>GQPPRRYTPDWPSLDSRPLPAWFDEAKFGVFIHWGVFSVPAWGSEWFWWHWQGEGRPQYQRFMRDNYPPGFSYADFGPQFTARFFHPEEWADLFQAAGAKYVVLTTKHHEGFTNWPSPVSWNWNSKDVGPHRDLVGELGTALRKRNIRYGLYHSLLEWFHPLYLLDKKNGFKTQHFVSAKTMPELYDLVNSYKPDLIWSDGEWECPDTYWNSTNFLSWLYNDSPVKDEVVVNDRWGQNCSCHHGGYYNCEDKFKPQSLPDHKWEMCTSIDKFSWGYRRDMALSDVTEESEIISELVQTVSLGGNYLLNIGPTKDGLIVPIFQERLLAVGKWLSINGEAIYASKPWRVQWEKNTTSVWYTSKGSAVYAIFLHWPENGVLNLESPITTSTTKITMLGIQGDLKWSTDPDKGLFISLPQLPPSAVPAEFAWTIKLTGVK[4x]

In humans, the dynamic process of α-L-fucose removal is catalyzed by two α-L-fucosidases—lysosomal FucA1 and secreted FucA2—both of which liberate α-L-fucose from fucosylated glycoconjugates. Here, we have used cryoelectron microscopy (cryo-EM) to determine the structure of human lysosomal α-L-fucosidase (FucA1) in both an unliganded state and in complex with the inhibitor deoxyfuconojirimycin. These structures, determined at 2.49 Å resolution, reveal the homotetrameric structure of FucA1, the architecture of the catalytic center, and the location of both natural population variations and disease-causing mutations. Each protomer of FucA1 is comprised of an N-terminal catalytic domain—a modified (β/α)8 barrel—and a C-terminal β-sandwich domain, which are characteristic of GH29 enzymes (Lombard et al., 2014).

To determine the structure of FucA1, we performed single-particle cryo-EM using a 200 kV Thermo Fisher Scientific Glacios electron cryo-microscope equipped with a Falcon-4 detector. Micrographs showed particles with diverse angular coverage, and secondary structural features could be observed in two-dimensional (2D) class averages. Further data processing resulted in a 3D reconstruction of FucA1 with dihedral symmetry (D2) and an overall resolution of 2.49 Å (see Figure S2 and Table 1 for data collection and refinement statistics). FucA1 forms a symmetric homotetramer approximately 150 × 100 × 40 Å in size. Each protomer interacts with two other protomers through residues in both the catalytic and β-sandwich domains, including the loop between residues 441 and 451, thus creating a flattened quaternary structure. We also observed cryo-EM density corresponding to one of the three predicted glycosylation sites. Many of the most frequent natural variants are present on external loops and α-helices; no active-site residues have any natural variation, and very few variants are present on the β-barrel core of the catalytic domain. Surprisingly, none of the missense mutations identified in cases of fucosidosis are present in the active site. The six known missense mutations represent either the shift from a non-polar residue to a charged residue in the protein’s interior (G60D, G340E, L405R) or a disruption of the hydrogen-bonding network of a polar residue by replacement with a non-polar/aromatic residue (S63L, S150F, N329Y).>[4x]MERQPTTDRMIQEYVPGKQVTLAHLIA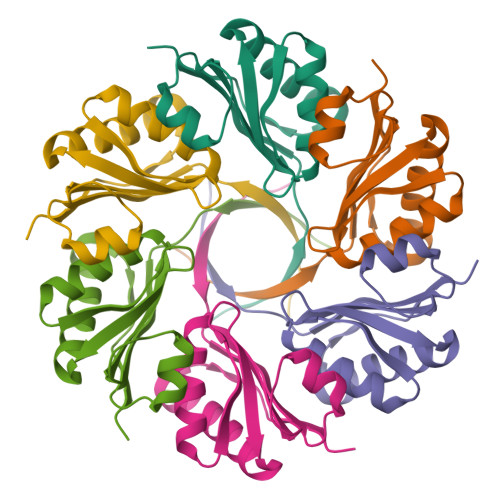NPGKDLFKKLGLQDAVSAIGILTITPSEASIIACDIATKSGAVEIGFLDRFTGAVVLTGDVSAVEYALKQVTRTLGEMMQFTTCSITRTLEHHHHHH1-BENZYL-1H-IMIDAZOLE | C10 H10 N2 | 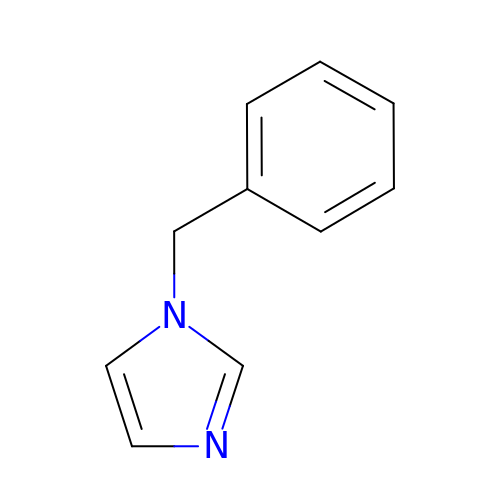KKKDZZRICRFGSD-UHFFFAOYSA-N>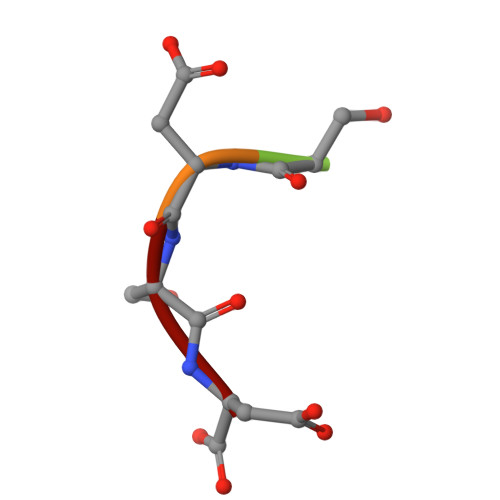 DSDSD> SEISRQEFQRRRQALVEQMQPGSAALIFAAPEVTRSADSEYPYRQNSDFWYFTGFNEPEAVLVLIKSDDTHNHSVLFNRVRDLTAEIWFGRRLGQDAAPEKLGVDRALAFSEINQQLYQLLNGLDVVYHAQGEYAYADVIVNSALEKLRKGSRQNLTAPATMIDWRP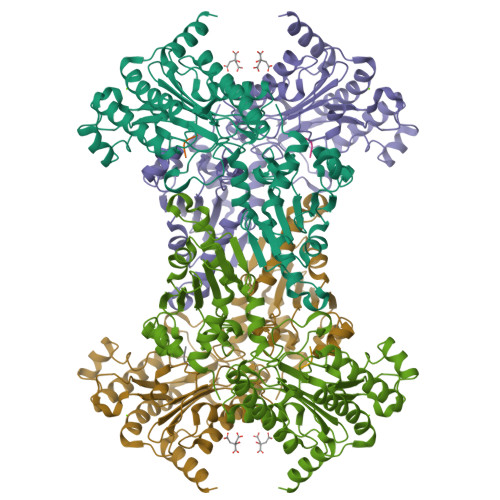VVHEMRLFKSPEEIAVLRRAGEITAMAHTRAMEKCRPGMFEYHLEGEIHHEFNRHGARYPSYNTIVGSGENGCILHYTENECEMRDGDLVLIDAGCEYKGYAGDITRTFPVNGKFTQAQREIYDIVLESLETSLRLYRPGTSILEVTGEVVRIMVSGLVKLGILKGDVDELIAQNAHRPFFMHGLSHWLGLDVHDVGVYGQDRSRILEPGMVLTVEPGLYIAPDAEVPEQYRGIGIRIEDDIVITETGNENLTASVVKKPEEIEALMVAARKQ;> VPL> IGVCYGMSANNLPAASTVVSMFKSNGIKSMRLYAPNQAALQAVGGTGINVVVGAPNDVLSNLAASPAAAASWVKS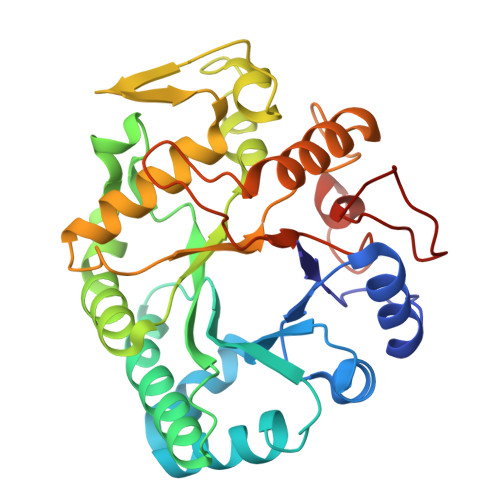NIQAYPKVSFRYVCVGNEVAGGATRNLVPAMKNVHGALVAAGLGHIKVTTSVSQAILGVFSPPSAGSFTGEAAAFMGPVVQFLARTNAPLMANIYPYLAWAYNPSAMDMGYALFNASGTVVRDGAYGYQNLFDTTVDAFYTAMGKHGGSSVKLVVSESGWPSGGGTAATPANARFYNQHLINHVGRGTPRHPGAIETYIFAMFNENQKDSGVEQNWGLFYPNMQHVYPINF> GAMDPEFGRPMEISDKISKEEMVRRLKMVVKTFMDMDQDSEEEKELYLNLALHLASDFFLKHPDKDVRLLVACCLADIFRIYAPEAPHTSPDKLKDIFMFITRQLKGLEDTKSPQFNRYFYLLENIAWVKSYNICFELEDSNEIFTQLYRTLFSVINNGHNQKVHMHMVDLMSSIICEGDTVSQELLDTVLVNLVPAHKNLNKQAYDLAKALLKRTAQAIEPYITNFFNQVLMLGKTSISDLSEHVFDLILELYNIDSHLLLSVLPQLEFKLKSNDNEERLQVVKLLAKMFGAKDSELASQNKPLWQCYLGRFNDIHVPIRLECVKFASHCLMNHPDLAKDLTEYLKVRSHDPEEAIRHDVIVSIVTAAKKDILLVNDHLLNFVRERTLDKRWRVRKEAMMGLAQIYKKYALQSAAGKDAAKQIAWIKDKLLHIYYQNSIDDRLLVERIFAQYMVPHNLETTERMKCLYYLYATLDLNAVKALNEMWKCQNLLRHQVKDLLDLIKQPKTDASVKAIFSKV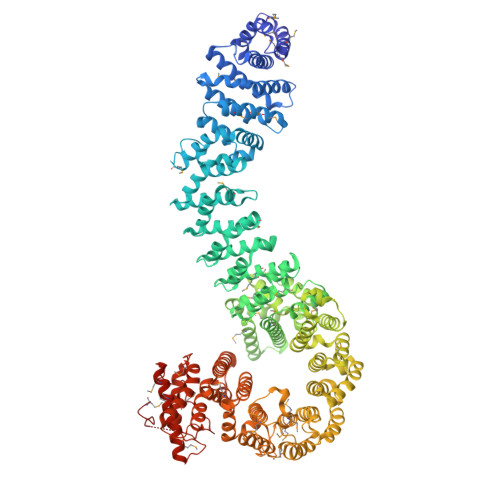MVITRNLPDPGKAQDFMKKFTQVLEDDEKIRKQLEVLVSPTCSCKQAEGCVREITKKLGNPKQPTNPFLEMIKFLLERIAPVHIDTESISALIKQVNKSIDGTADDEDEGVPTDQAIRAGLELLKVLSFTHPISFHSAETFESLLACLKMDDEKVAEAALQIFKNTGSKIEEDFPHIRSALLPVLHHKSKKGPPRQAKYAIHCIHAIFSSKETQFAQIFEPLHKSLDPSNLEHLITPLVTIGHIALLAPDQFAAPLKSLVATFIVKDLLMNDRLPGKKTTKLWVPDEEVSPETMVKIQAIKMMVRWLLGMKNNHSKSGTSTLRLLTTILHSDGDLTEQGKISKPDMSRLRLAAGSAIVKLAQEPCYHEIITLEQYQLCALAINDECYQVRQVFAQKLHKGLSRLRLPLEYMAICALCAKDPVKERRAHARQCLVKNINVRREYLKQHAAVSEKLLSLLPEYVVPYTIHLLAHDPDYVKVQDIEQLKDVKECLWFVLEILMAKNENNSHAFIRKMVENIKQTKDAQGPDDAKMNEKLYTVCDVAMNIIMSKSTTYSLESPKDPVLPARFFTQPDKNFSNTKNYLPPEMKSFF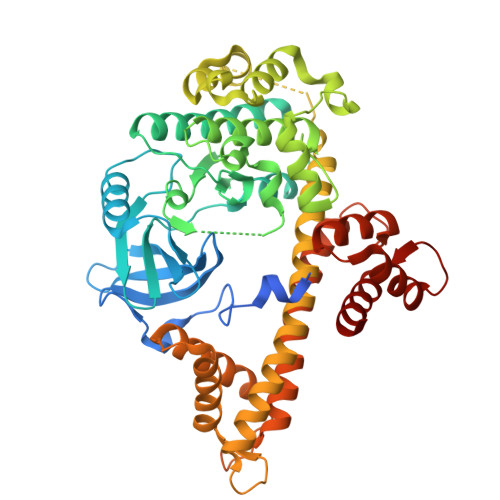> GNTKNEHHKTNKKSLKGGNERHEMKESSVGISKKIVENSFNNSKLRPGMFIQNSNVVFNEQYKGIKILGKGSFGEVILSRDKHTGHEYAIKVISKKHVKRKTDKESLLREVELLKMLDHINIMKLYEFFEDNNYYYLVSDVYTGGELFDEIISRKRFYEIDAARIIKQILSGITYMHKNNVVHRDLKPENILLETKNKEDMIIKIIDFGLSTHFEYSKKMKDKIGTAYYIAPDVLHGTYDEKCDIWSCGVILYILLSGCPPFNGSNEYDILKKVEAGKYTFDLPQFKKISDKAKDLIKKMLMYTSAVRISARDALEHEWIKMMTSKDNLNIDIPSLELSIANIRQFQSTQKLAQAALLYMGSKLTTIDETKELTKIFKKMDKNGDGQLDRNELIIGYKELLKLKGEDTSDLDNAAIEYEVDQILNSIDLDQNGYIEYSEFLTVSIDRKLLLSTERLEKAFKLFDKDGSGKISANELAQLFGLSDVSSECWKTVLKEVDQNNDGEIDFKEFRDMLVKLCNY>NAQFLHTQVGRGLLGAVVNPLGEVTDKFAVTDNSEILYRPVDNAPPLYSERAAIEKPFLTGIKVIDSLLTCGEGQRMGIFASAGCGKTFLMNMLIEHSGADIYVIGLIGERGREVTETVDYLKNSEKKSRCVLVYATSDYSSVDRCNAAYIATAIAEFFRTEGHKVALFIDSLTRYARALRDVALAAGRSPARRGYPVSVFDSLPRLLERPGKLKAGGSITAFYTVLLEDDDFADPLAEEVRSILDGHIYLSRNLAQKG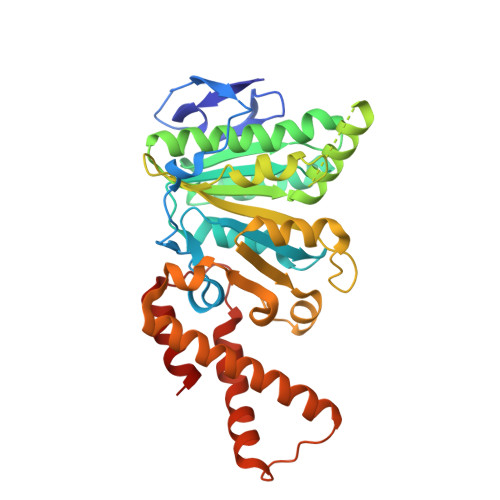QFPAIDSLKSISRVFTQVVDEKHRIMAAAFRELLSEIEELRTIIDFGEYKPGENASQDKIYNKISVVESFLKQDYRLGFTYEQTMELIGETIR[2x]> MDEEQPPIERVDYICERSVVVPVTYIRSNGAPAAAVLEVEGKMVALQWHGDLKKYVAIDEQDSYRWADRGGQATLSHLEADHT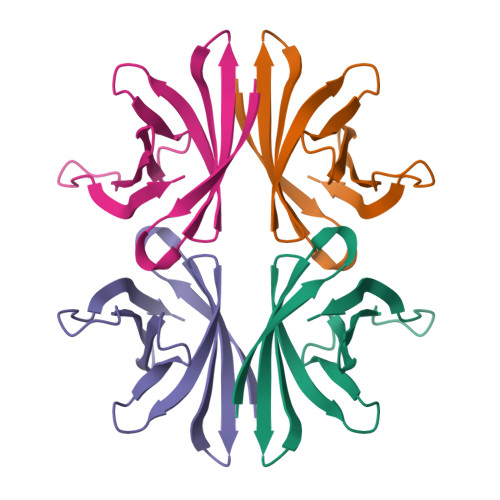AKEVTLLSACRADTAEELEHHHHHH> EDEDGDYEELVLALRSEEDGLAEAPEHGTTATFHRCAKDPWRLPGTYVVVLKEETHLSQSERTARRLQAQAARRGYLT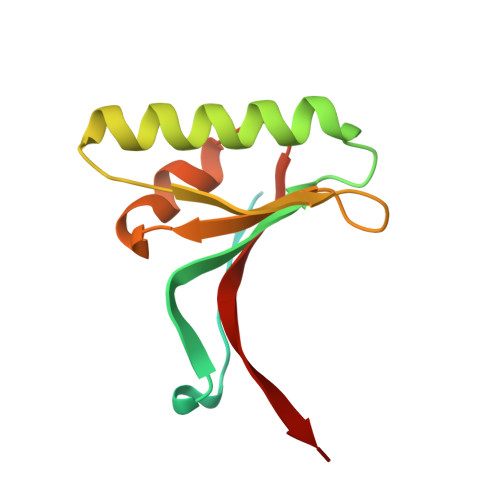KILHVFHGLLPGFLVKMSGDLLELALKLPHVDYIEEDSSVFAQ> GSQDLQLVKGAMAAT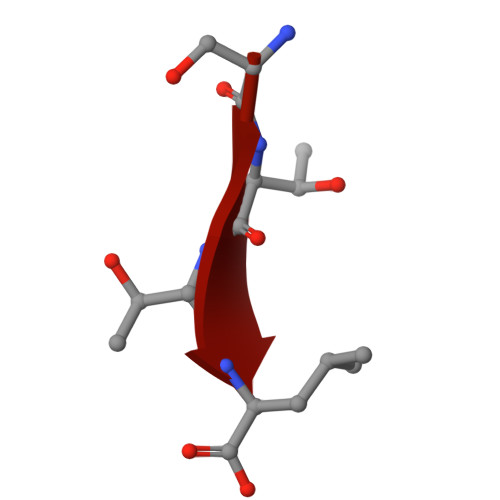YSALNSSKPTPQLKPIESSILAQRRVRKLPSTTL> MRSRTANRSGIVIRRRVTPAGDIIVTLLTPQGKLKAIARGGVKGPLSSSLNLFHHVGVQVYQGPHNDLASVKQAVLEGALPTLAEPERYAFAHLMAEFADALFQEGEFSEQAFDLFAASLRGVAHQPDPEWVALVMSYKLLGLAGVIPQTARCARCGAPDPEHPDPLGGQLLC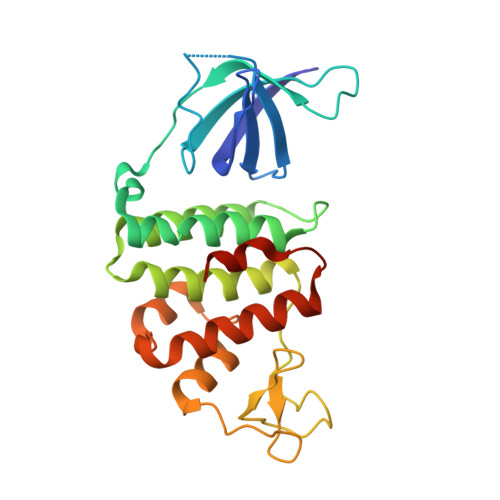SKCAALPPYPPAVLDFLRHAVRRTVRASFEQPVPSADRPALWRALEKFVTVQVGGVHSWRQLVPSGVPVLS>[8x]MLSGLNHLTLAVSQLAPSVAFYQQLLGMTLHARWDSGAYLSCGDLWLCLSLD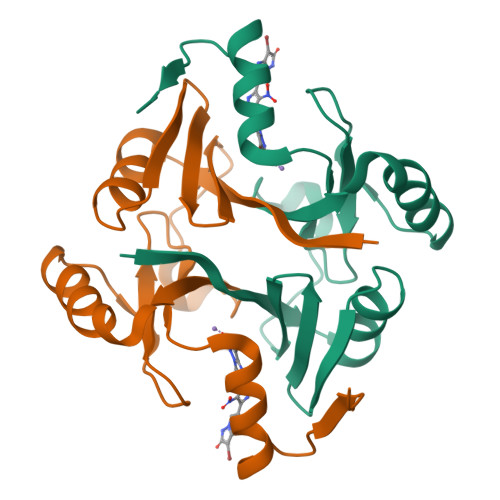PQRRVTPPEESDYTHYAFSISEADFASFAARLEAAGVAVWKLNRSEGASHYFLDPDGHKLELHVGSLAQRLAACREQPYKGMVFFEQHHHHHH2,2'-{[9-(HYDROXYIMINO)-9H-FLUORENE-2,7-DIYL]BIS(OXY)}DIACETIC ACID | C17 H13 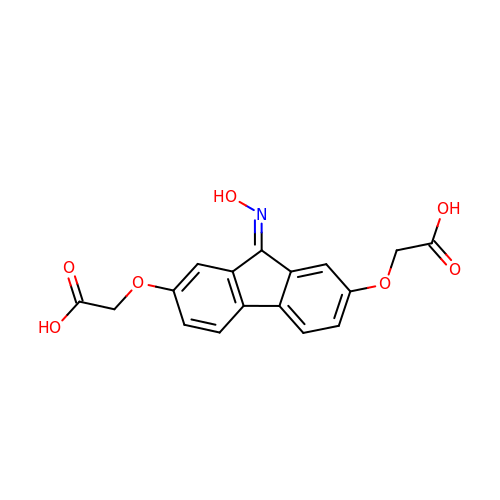N O7 | VOKATEXROYSXDW-UHFFFAOYSA-N>[2x]MLSQTLLEMTEQMIEVAEKGADRYQEGKNSNHSYDFFETIKPAVEENDELAARWAEGALELIKVRRPKYVHKEQIEAVKDNFLELVLQSYVHHIHKKRFKDITESVLYTLHAVKD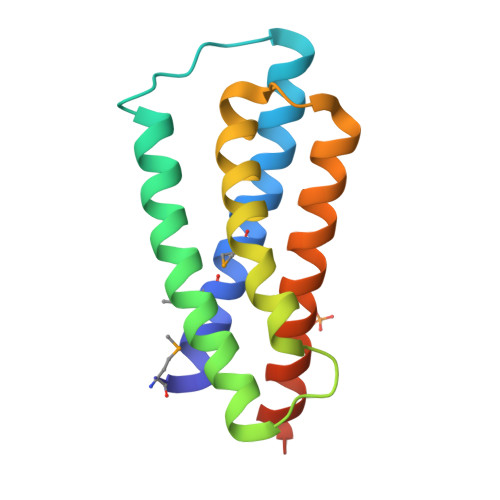EIAREDSRLEHHHHHH3-[decyl(dimethyl)ammonio]propane-1-sulfonate 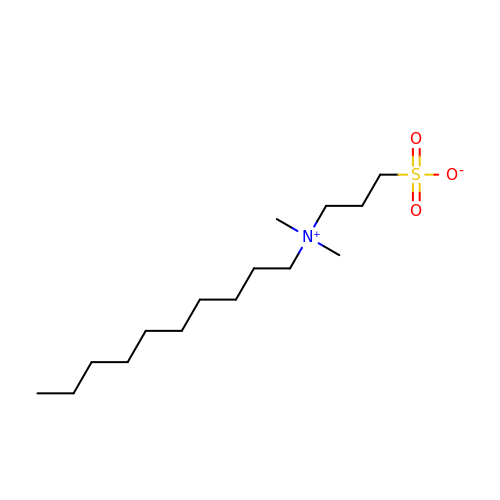| C15 H33 N O3 S | WKALLSVICJPZTM-UHFFFAOYSA-N> QGSCMSITINPSRPSVNNIGQVDIDSVILGRPGAIGSW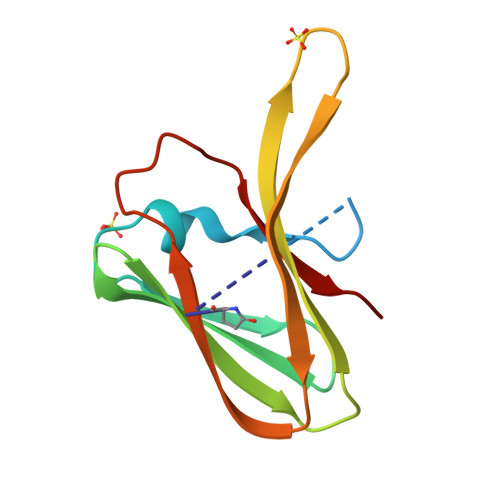ELNNFITIGLNRVNADTVRVNIRNTGRTNRLIITQWDNTVTRGDVYELFGDYALIQGRGSFCLNIRSDTGRENWRMQLEN> 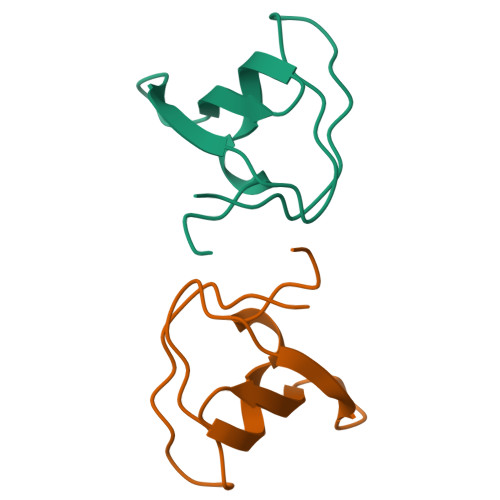MNDPNLFVALYDFVASGDNTLSITKGEKLRVLGYNHNGEWCEAQTKNGQGWVPSNYITPVNS> TDTFQMFWLDYCEVNNTLILFGKVKLKDDNCVSAMVQINGLCRELFFLPREGKTPTDIHEEIIPLLMDKYGLDNIRAKPQKMKYSFELPDIPSESDYLKVLLPYQTPKSSRDTIPSDLSSDTFYHVFGGNSNIFESFVIQNRIMGPCWLDIKGADFNSIRNASHCAVEVSVDKPQNITPTTTKTMPNLRCLSLSIQTLMNPKENKQEIVSITLSAYRNISLDSPIPENIKPDDLCTLVRPPQSTSFPLGLAALAKQKLPGRVRLFNNEKAMLSCFCAMLKVEDPDVIIGHRLQNVYLDVLAHRMHDLNIPTFSSIGRRLRRTWPEKFGRGNSNMNHFFISDICSGRLICDIANEMGQSLTPKCQSWDLSEMYQV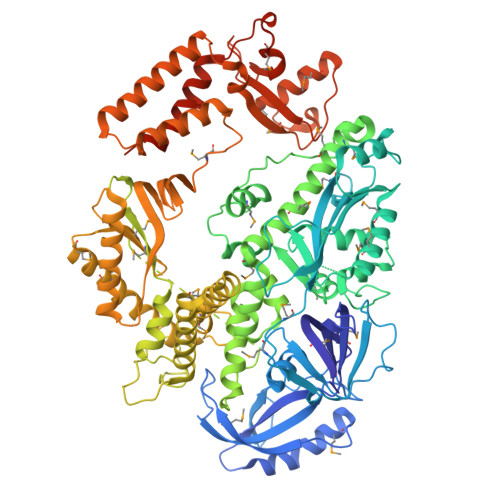TCEKEHKPLDIDYQNPQYQNDVNSMTMALQENITNCMISAEVSYRIQLLTLTKQLTNLAGNAWAQTLGGTRAGRNEYILLHEFSRNGFIVPDKEGNRSRAQKQRQNEENADAPVNSKKAKYQGGLVFEPEKGLHKNYVLVMDFNSLYPSIIQEFNICFTTVDRNKEDIDELPSVPPSEVDQGVLPRLLANLVDRRREVKKVMKTETDPHKRVQCDIRQQALKLTANSMYGCLGYVNSRFYAKPLAMLVTNKGREILMNTRQLAESMNLLVVYGDTDSVMIDTGCDNYADAIKIGLGFKRLVNERYRLLEIDIDNVFKKLLLHAKKKYAALTVNLDKNGNGTTVLEVKGLDMKRREFCPLSRDVSIHVLNTILSDKDPEEALQEVYDYLEDIRIKVETNNIRIDKYKINMKLSKDPKAYPGGKNMPAVQVALRMRKAGRVVKAGSVITFVITKQDEIDNAADTPALSVAERAHALNEVMIKSNNLIPDPQYYLEKQIFAPVERLLERIDSFNVVRLSEALGLDSKKYFRREGGNNNG> MLRSLLQSGHRRVVASSCATMVRCSSSSTSALAYKQMHRHATRPPLPTLDTPSWNANSAVSSIIYETPAPSRQPRKQHVLNCLVQNEPGVLSRVSGTLAARGFNIDSLV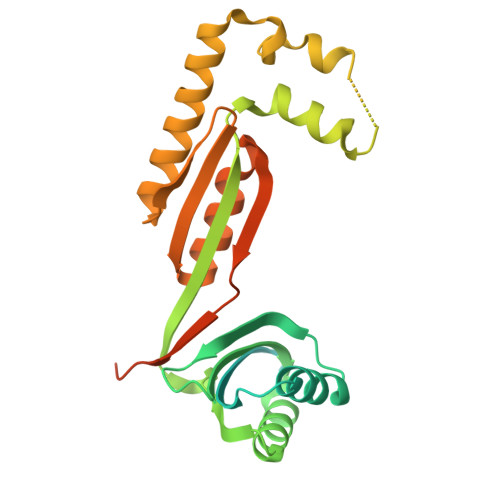VCNTEVKDLSRMTIVLQGQDGVIEQARRQIEDLVPVYAVLDYTNSEIIKRELVMARISLLGTEYFEDLLLHHHTSTNAGAADSQELVAEIREKQFHPANLPASEVLRLKHEHLNDITNLTNNFGGRVVDISETSCIVELSAKPTRISAFLKLVEPFGVLECARSGMMALPRTPLKTSTEEAADEDEKISEIVDISQLPPG> MSRQVVRSSKFRHVFGQPAKADQCYEDVRVSQTTWDSGFCAVNPKFMALICEASGGGAFLVLPLGKTGRVDKNVPLVCGHTAPVLDIAWCPHNDNVIASGSEDCTVMVWEIPDGGLVLPLREPVITLEGHTKRVGIVAWHPTAQNVLLSAGCDNVILVWDVGTGAAVLTLGPDVHPDTIYSVDWSRDGALICTSCRDKRVRVIEPRKGTVVAEKDRPHEGT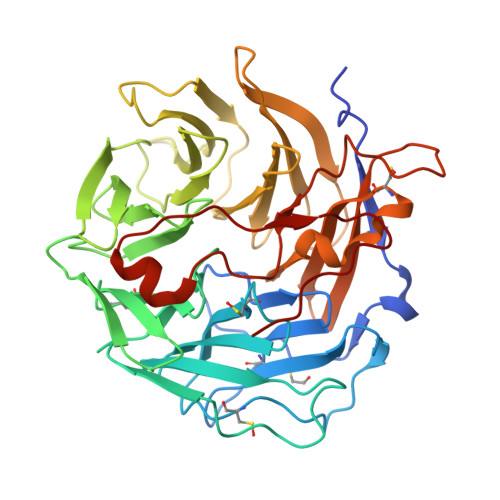RPVHAVFVSEGKILTTGFSRMSERQVALWDTKHLEEPLSLQELDTSSGVLLPFFDPDTNIVYLCGKGDSSIRYFEITSEAPFLHYLSMFSSKESQRGMGYMPKRGLEVNKCEIARFYKLHERKCEPIAMTVPRKSDLFQEDLYPPTAGPDPALTAEEWLGGRDAGPLLISLKDGYVPPKSR>MRLTKFTDLALRSLMRLAVVRDGDEPLATREVAEVVGVPYTHAAKAITRLQHLGVVEARRGRGGGLT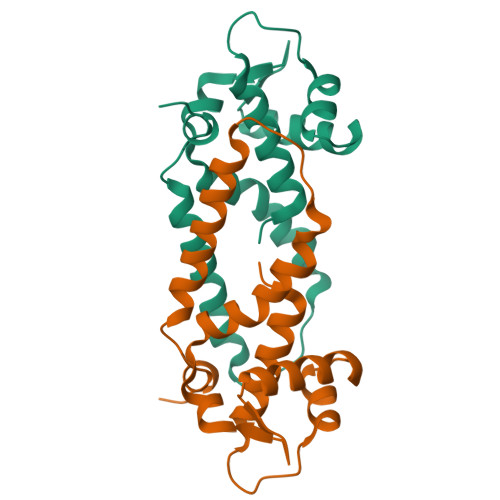LTDLGRRVSVGWLVRELEGEAEVVDAEGDNPAPLRGAARLRRALRDAQEAFYAALDPLTVTDLVAAPTGPVLLGLTDRPSGKLAAALEHHHHHH[5x]> GPGGSMKRLRPSDKFFELLGYKPHHVQLAIHRSTAKRRVACLGRQSGKSEAASVEAVFELFARPGSQGWIIAPTYDQAEIIFGRVVEKVERLAEVFPATEVQLQRRRLRLLVHHYDRPVNAPGAKRVATSEFRGKSADRPDNLRGATLDFVILDEAAMIPFSVWSEAIEPTL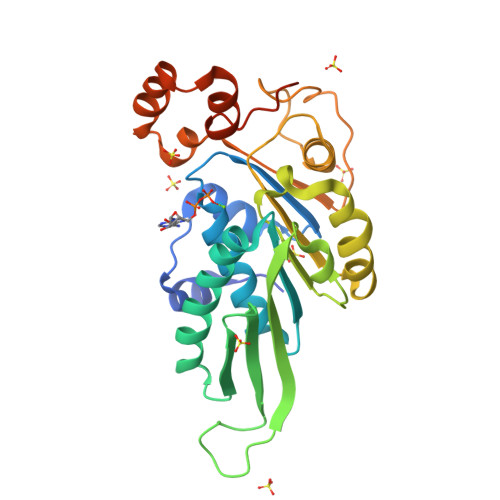SVRDGWALIISTPKGLNWFYEFFLMGWRGGLKEGIPNSGINQTHPDFESFHAASWDVWPERREWYMERRLYIPDLEFRQEYGAEFVSHSGLEHHHHHHHHHH>VNTNIASLNTQRNLNASSNDLNTSLQRLTTGYRINSAKDDAAGLQISNRLSNQISGLNVATRNANDGISLAQTAEGALQQSTNILQRIRDLALQSANGSNSDADRAALQKEVAAQQAELTRISDTTTFGGRKLLDGSFGTTSFQVGSNAYETIDISLQNASASAIGSYQVGSNGAGTVASVAGTATASGIASGTVNLVGGGQVKNIAIAAGDSAKAIAEKMDGAIPNLSARARTVFTADVSGVTGGSLNFDVTVGSNTVSLAGVTSTQDLADQLNSNSSKLGITASINDKGVLTITSATGENVKFGAQTGTATAGQVAVKVQGSDGKFEAAAKNVVAAGTAATTTIVTGYVQLNSP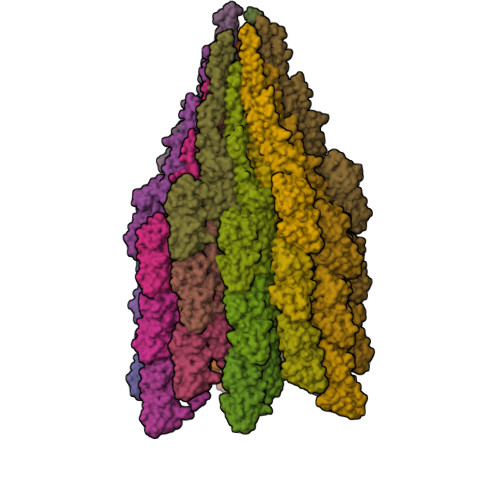TAYSVSGTGTQASQVFGNASAAQKSSVASVDISTADGAQNAIAVVDNALAAIDAQRADLAAVQNRFKNTIDNLTNISENATNARSRIKDTDFAAETAALSKNQVLQQAGTAILAQANQLPQAVLSLLR[33x]> PALPEDGGSGAFPPGHFKDPKRLYCKNGGFFLRIHPDGRVDGVREKSDPHIKLQLQAEERGVVSIKGVCANRYLAMKEDGRLLASK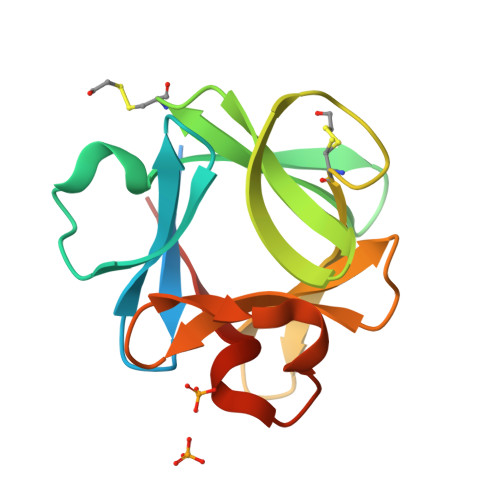CVTDECFFFERLESNNYNTYRSRKYTSWYVALKRTGQYKLGSKTGPGQKAILFLPMSAKS> SDDVVTFKAQEQLQRASEQAHNSPVLRALLAESLRLFEQVAGSLTPANLTTAVEQYISLKYYAGAIQLCLTVAQQKDRGNTALSWVNDGKPANDSRKKAFDERKICYNLIHQVLDKLESDFAGEPELVDGRPTLAATKRMEAYNVVNDSSDE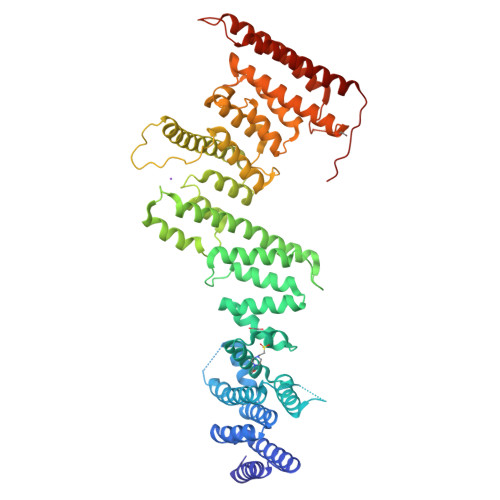VFHFDLYEWYIEKGWTDRILSIDSPHVITYLQRLAETDFRHAELLCRFYTTRSRFFEAAQVQTNLAKSDLNISLKDRIILLSRAKGNASVNTIGISRQQQQQLNHEASELLEIAHIQDDLLERLVADPRIPEERKAEIEEFLDGPIRTLTDLFNDYADQANYYDLCLLIFHAADFHNPRTILDTWNNLINQSHFEAEQRREYWEIVQAGGDLPAGVIAPIAEPPLPYVYVSQQIQLIAHRTSLDSLIFPVNSLLPVVCAYAINNGQDASIGADPCWPIQLFLNLGVPHALVVQVLENVLDTQEAPFTGRRRKLVVQWIAMAVDMWVREVERRGAMAAAAASGASGSEAVMGSWVSELLGRADQVLTQIAGTGATLRGGAASDAEEIASLRRTVKGLKRSVDMLLGGEMARMSFFR>MNNYVKVHQPLNVDLRTQKTQTKLYTVLERFYVEDRTFESISIKDLC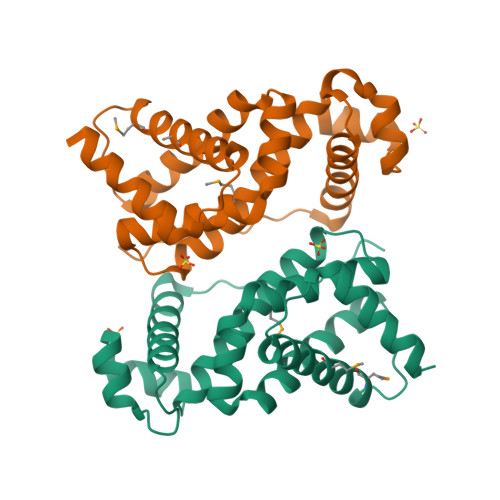EQARVSRATFYRHHKEIIQVIEVQILRTMQYFSLEFDQIILTKENIQRLILRTIQKNPLLFQVIFWSRAENIFIDVVSGEILRISLLKEVSFSDSKFMPNCFARMILSLAAEIQQSNKDYTNDQLVELIQEAARFLQK[2x]> WGQGTLVTVSAESARNPTIYPLTLPPALSSDPVIIGCLIHDYFPSGTMNVTWGKSGKDITTVNFPPALASGGRYTMSSQLTLPAVECPEGESVKCSVQHDSNPVQELDVNCSGPTPPPPITIPSCQPSLSLQRPALEDLLLGSDASITCTLNGLRNPEGAVFTWEPSTGKDAVQK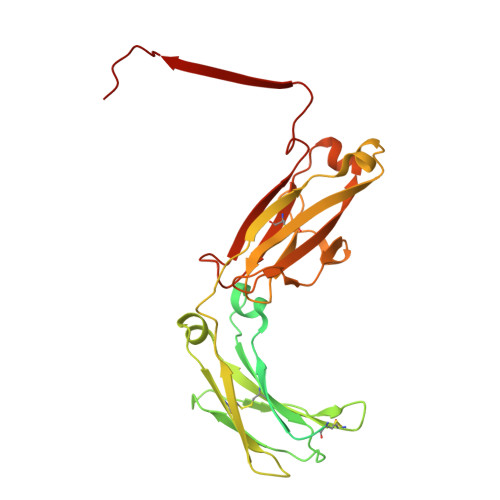KAVQNSCGCYSVSSVLPGCAERWNSGASFKCTVTHPESGTLTGTIAKVTVNTFPPQVHLLPPPSEELALNELLSLTCLVRAFNPKEVLVRWLHGNEELSPESYLVFEPLKEPGEGATTYLVTSVLRVSAETWKQGDQYSCMVGHEALPMNFTQKTIDRLSGKPTNVSVSVIMSEGDGICY N-[(1S,2R)-1-benzyl-2-hydroxy-3-{[3-(trifluoromethyl)benzyl]amino}propyl]-3-(1,1-dioxido-1,2-thiazinan-2-yl)-5-(ethylamino)benzamide 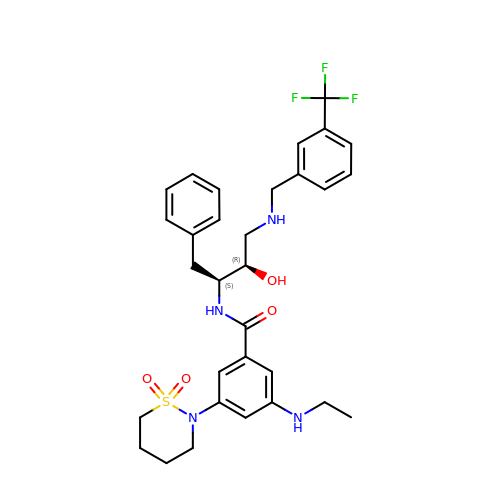| C31 H37 F3 N4 O4 S | GPMRAYXRPZKTFK-URLMMPGGSA-N> MTNQQEQHIAIFTTASI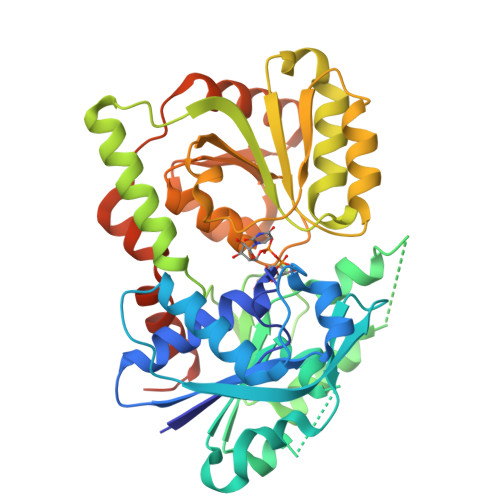PWLTGTAVNPLFRAAYLANDGERRVTLVIPWLTLKHQKLVYPNSITFSSPSEQEAYVRQWLEERVSFRLAFEIRFYPGKFAIDKRSILPVGDISDAIPDEEADIAVLEEPEHLTWFHHGQKWKTKFNYVIGIVHTNYLEYVKREKQGRVKAFFLKYLNSWVVGIYCHKVIRLSAATQEYPKSIVCNVHGVNPKFLEIGLRKLEQQKLQEQPFTKGAYYIGKMVWSKGYKELLKLLEKHQKELAELEVDLYGDGEDSEEIKEAARKLDLTVNVYPGRDHADSLFHNYKVFLNPSTTDVVCTTTAEALAMGKIVVCANHISNKFFKQFPNCRTYDDGQGFVRATLKALGEQPSQLTEQQRHELSWEAATQRFIKVSDLNRLSRADKLAAHHHHHHHH> MGSSHHHHHHSQDPMSMTILPLELIDKCIGSNLWVIMKSEREFAGTLVGFDDYVNIVLKDVTEYDTVTGVTEKHSEMLLNGNGMCMLIPGGKPE;> MDSSPNEFLNKVIGKKVLIRLSSGVDYKGILSCLDGYMNL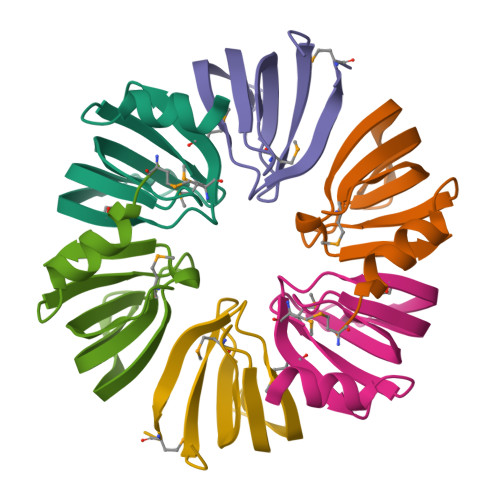ALERTEEYVNGKKTNVYGDAFIRGNNVLYVSALDD;> MSSLQKRPGPGNSSQPTERPRKESILDLSRYQDQRIQATFTGGRQITGILKGFDQLMNLVLDDVEEQLRNPEDGKLTGAIRKLGLVVVRGTTLVLIAPMDGSEEIPNPFVQAE1-[(4S)-2,5-DIOXOIMIDAZOLIDIN-4-YL]UREA | C4 H6 N4 O3 | 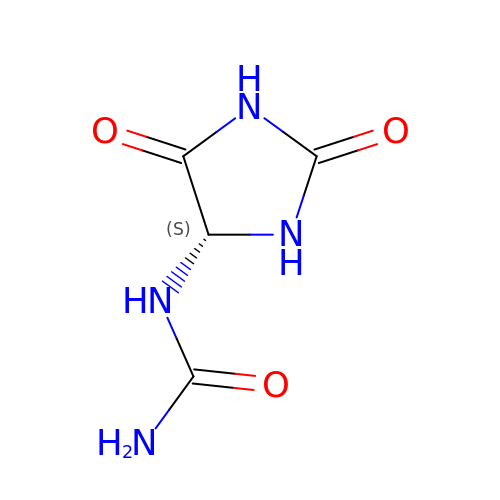POJWUDADGALRAB-SFOWXEAESA-N> SLSTIICIGMAGSGKTTFMQRLNSHLRAEKTPPYVINLDPAVLRVPYGANIDIRDSIKYKKVMENYQLGPNGAIVTSLNLFSTKIDQVIRLVEQKKDKFQNCIIDTPGQIECFVWSASGAIITESFASSFPTVIAYIVDTPRNSSPTTFMSNMLYACSILYKTKLPMIVVFNKTDVCKADFAKEWMTDFESFQAAIKEDQDG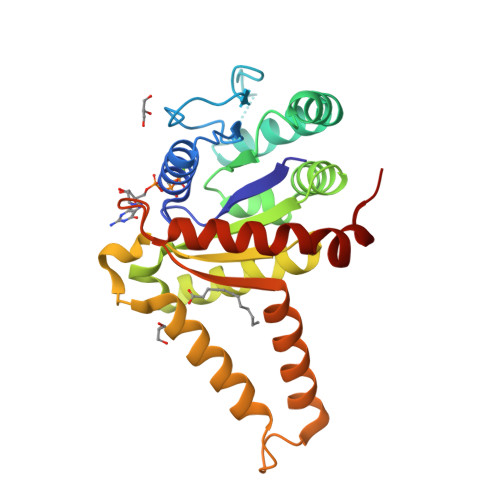YMSSLVNSMSLMLEEFYSQLDVVGVSSFTGDGFDEFMQCVDKKVDEYDQYYKKHHHHHH>[4x]VDSKKRPGKDLDRIDRNILNELQKDGRISNVELSKRVGLSPTP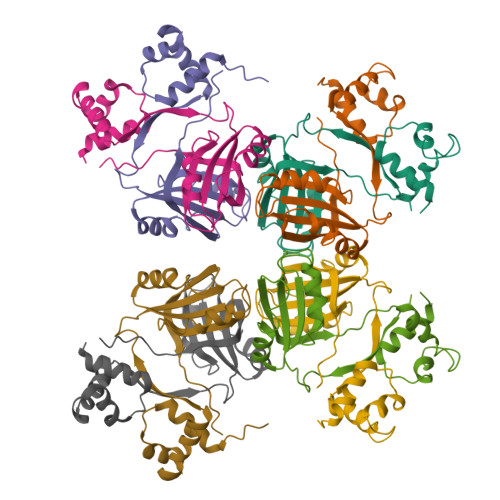CLERVRRLERQGFIQGYTALLNPHYLDASLLVFVEITLNRGAPDVFEQFNTAVQKLEEIQECHLVSGDFDYLLKTRVPDMSAYRKLLGETLLRLPGVNDTRTYVVMEEVKQSNRLVIKTR>MSYPEKFEGIAIQSHEDWKNPKKTKYDPKPFYDHDIDIKIEACGVCGSDIHCAAGHWGNMKMPLVVGHEIVGKVVKLGPKSNSGLKVGQRVGVGAQVFSCLECDRCKNDNEPYCTKFVTTYSQPYEDGYVSQGG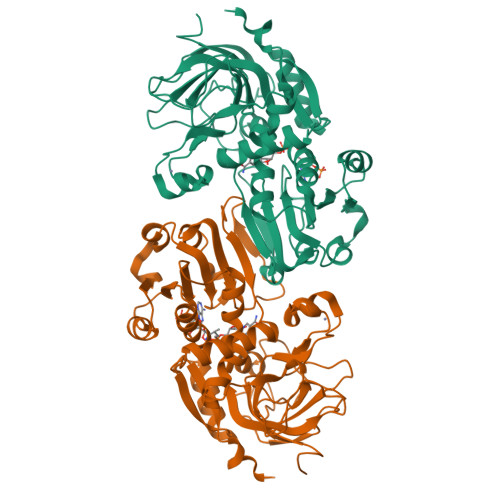YANYVRVHEHFVVPIPENIPSHLAAPLLCGGLTVYSPLVRNGCGPGKKVGIVGLGGIGSMGTLISKAMGAETYVISRSSRKREDAMKMGADHYIATLEEGDWGEKYFDTFDLIVVCASSLTDIDFNIMPKAMKVGGRIVSISIPEQHEMLSLKPYGLKAVSISYSALGSIKELNQLLKLVSEKDIKIWVETLPVGEAGVHEAFERMEKGDVRYRFTLVGYDKEFSD[2x]>MGVDPFERNKILGRGINIGNALEAPNEGDWGVVIKDEFFDIIKEAGFSHVRIPIRWSTHAYAFPPYKIMDRFFKRVDEVINGALKRGLAVVINIHHYEELMNDPEEHKERFLALWKQIADRYKDYPETLFFEILNEPHGNLTPEKWNELLEEALKVIRSIDKKHTI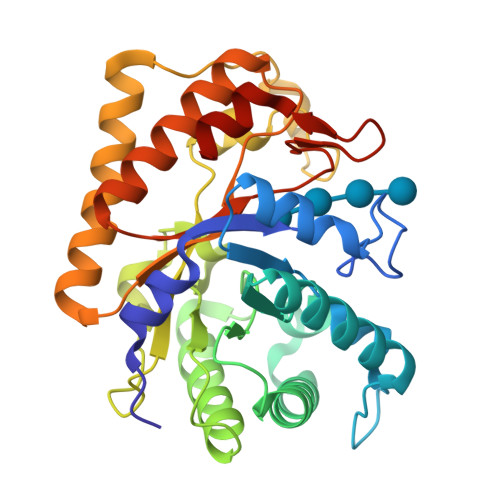IIGTAEWGGISALEKLSVPKWEKNSIVTIHYYNPFEFTHQGAEWVEGSEKWLGRKWGSPDDQKHLIEEFNFIEEWSKKNKRPIYIGAFGAYRKADLESRIKWTSFVVREMEKRRWSWAYWEFCSGFGVYDTLRKTWNKDLLEALIGGDSIE[4x]>GPLGSMPGEEEERAFLVAREELASALRRDSGQAFSLEQLRPLLASSLPLAARYLQLDAARLVRCNAHGEPRNYLNTLSTALNILEKYGRNLLSPQRPRYWRGVKFNNPVFRSTVDAVQGGRDVLRLYGYTEEQPDGLSFPEGQEEPDEHQVATVTLEVLLLRTELSLLLQNTHPRQQALEQLLE[2x];>FTDCQLAAAVCMTY[2x]

To target disease-causing proteins that are inaccessible to small-molecule or antibody therapies, we are exploring the use of a nature-inspired drug modality that exploits the intrinsically favorable properties of synthetically constrained α-helical polypeptides (Helicons). Here, we report a rapid, high-throughput screening platform utilizing phage display that enables an unbiased mapping of the α-helical interactome of a given protein without any prior knowledge of its structure or known binding partners. Analysis of 14 high-resolution crystal structures of Helicon–protein complexes across six different protein domains reveals a range of binding modes, all of which are “side-on”, i.e., mediated exclusively by Helicon side-chains rather than involving main chain amide interactions. Biochemical and structural experiments demonstrate diverse functional impacts by the Helicons which bind these sites, including inhibition of protein–protein interactions, inhibition of enzymatic activity, induced conformational rearrangement, and induced dimerization.

We began with the E3 ubiquitin ligase RNF31, which is an integral component of the linear ubiquitin chain assembly complex. RNF31 is a 1,072-amino acid protein comprised of multiple folded and disordered regions. We screened two of the nonenzymatic folded domains, the PUB and UBA domains, each at multiple concentrations and in the presence or absence of a known binding partner. Most hits for the RNF31 PUB domain could be grouped into two families of related clusters (C41 to C43 and C44 to C45), both of which competed with the natural binding partner Otulin, and both of which appeared to contain a critical tyrosine residue – also found in Otulin – but that had otherwise dissimilar logos. Upon solving X-ray cocrystal structures of member from a representative cluster of each family, we found that two Helicons, FP06649 from Cluster C44 and FP06652 from C41, bound the same site at the protein surface, but that they engaged this site using completely different binding modes, with the critical tyrosine residues oriented differently. This observation was our first structural evidence of the ability of Helicons to identify distinct binding solutions to a common site, which we have since observed for several other target proteins.>REVLTGGHSVSAPQENRIYVMDSVFMHLTESRVHVYDYTNGKFLGMVPTAFNGHVQVSNDGKKIYTMTTYHERITRGKRSDVVEVWDADKLTFEKEISLPPKRVQGLNYDGLFRQTTDGKFIVLQNASPATSIGIVDVAKGDYVEDVTAAAGCWSVIPQPNRPRSFMTICGDGGLLTINLGEDGKVASQSRSKQMFSVKDDPIFIAPALDKDKAHFVSYYGNVYSADFSGDEVKVDGPWSLLNDEDKAKNWVPGGYNLVGLHRASGRMYVFMHPDGKEGTHKFPAAEIWVMDTKTKQRVARIPGRDALSMTIDQQRNLMLTLDGGNVNVYDISQPEPKLLRTIEGAAEASLQVQFHPVGGV[2x];>[2x]HISLNPDLANEDEVNSCDYWRHCAVDGFLCSCCGGTTTTCP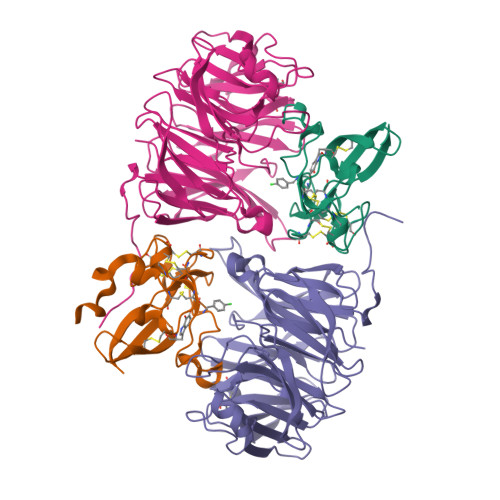PGSTPSPISWIGTCHNPHDGKDYLISYHDCCGKTACGRCQCNTQTRERPGYEFFLHNDVNWCMANENSTFHCTTSVLVGLAKN> MSKLEAILSQEVEAEIQALLQEAEAKAEAVKREAEEKAKALLQARERALEAQYRAALRRAESAGELLVATARTQARGEVLEEVRRRVREALEALPQKPEWPEVVR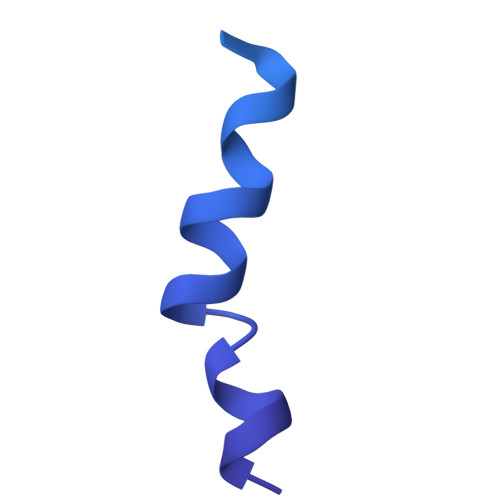KLALEALEALPGAKALVANPEDLPHLEALARERGVELQAEPALRLGVRAVGAEGKTQVENSLLARLDRAWDALSSKVAQALWG> XADVAGTSNRDFRGREQRLFNSEQYNYNNSLNG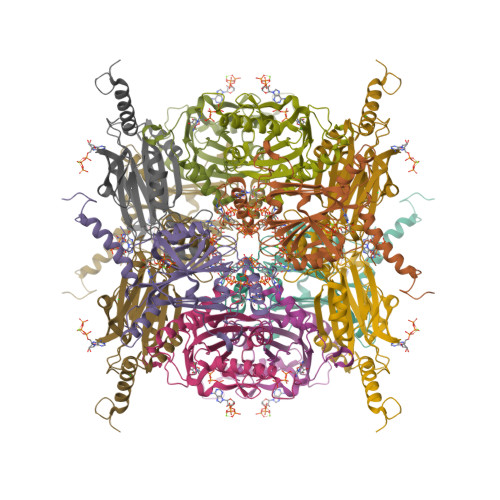EVSVWVYAYYSDGSVLVINKNSQYKVGISETFKALKEYRKGQHNDSYDEYEVNQSIYYPNGGDARKFHSNAKPRAIQIIFSPSVNVRTIKMAKGNAVSVPDEYLQRSHPWEATGIKYRKIKRDGEIVGYSHYFELPHEYNSISLAVSGVHKNPSSYNVGSAHNVMDVFQSCDLALRFCNRYWAELELVNHYISPNAYPYLDINNHSYGVALSNRQ Transient receptor potential vanilloid (TRPV) channels are a group of six polymodal cation channels subdivided into two subgroups by their sequence identity and functional properties. TRPV1–TRPV4 comprise the first subgroup of non-selective Ca2+ channels, TRPV5 and TRPV6 constitute the second subgroup of Ca2+ selective channels. TRPV channels are blocked by ruthenium red (RR), a universal pore blocker for a wide array of cation channels. Here we use cryo-electron microscopy to reveal the molecular details of RR block in TRPV2 and TRPV5, members of the two TRPV subfamilies.

Next, we prepared cryo-EM grids of wild-type rat TRPV2 reconstituted into nanodiscs in the presence of 1 mM of the robust TRPV2 activator 2-APB and 1 mM RR. Therefore, we used a high concentration of RR to ensure saturation. This dataset yielded a single stable high-quality state: 2-APB-activated RR-blocked TRPV2 (TRPV22APB+RR) with C4 symmetry at 2.9 Å resolution. The strong extra density at the TRPV22APB+RR SF was clearly visible from early stages of data processing before application of any symmetry and is aligned along the central symmetry axis; the size and shape of this density is consistent with the expected dimensions for RR and density consistent with 2-APB is present at our previously proposed 2-APB binding site and not in the vanilloid pocket (Pumroy et al, 2022). The SF of TRPV22APB+RR has adapted to accommodate RR, with tight coordination by the backbone carbonyl of Gly606 along the interior of the SF and the lower gate is closed at Met645. The primary site for RR stabilization in TRPV22APB+RR is the carbonyl of Gly606, which at distances of 3.0–3.2 Å can form hydrogen bonds with ammonia groups coordinated to the central and bottom ruthenium atoms. Additionally, density for the top ruthenium atom was more poorly resolved than the lower two ruthenium atoms, indicating that the top ruthenium group is not tightly coordinated. The only significant conformational difference between TRPV22APB+RR and TRPV22APB_AC is at the pore, where a downward rotation (9°) and shift (1.1 Å) of the pore helix to accommodate RR leads to subtle shifts in S5 and S6 which constrict the lower gate at Met645. The rest of the channel maintained the previously observed activated conformation, where the C-terminus is in a helical conformation rather than the loop conformation seen in the inactivated state (Pumroy et al, 2022). Our TRPV22APB+RR structure revealed that binding of RR to the 2-ABP-activated TRPV2 stabilized the channel in an intermediate conformation, preventing ion flow through the occluded SF and closing the lower gate at Met645, but at the same time inhibiting the transition to the inactivated state. This TRPV2 locked in an activated conformation allowed us to resolve clear density for 2-APB in our previously proposed 2-APB binding site, but not in the vanilloid pocket, a recently suggested alternate 2-APB site in mouse TRPV2.

>MTSASSPPAFRLETSDGDEEGNAEVNKGKQEPPPMESPFQREDRNSSPQIKVNLNFIKRPPKNTSAPSQQEPDRFDRDRLFSVVSRGVPEELTGLLEYLRWNSKYLTDSAYTEGSTGKTCLMKAVLNLQDGVNACIMPLLQIDKDSGNPKLLVNAQCTDEFYQGHSALHIAIEKRSLQCVKLLVENGADVHLRACGRFFQKHQGTCFYFGELPLSLAACTKQWDVVTYLLENPHQPASLEATDSLGNTVLHALVMIADNSPENSALVIHMYDGLLQMGARLCPTVQLEEISNHQGLTPLKLAAKEGKIEIFRHILQREFSGPYQPLSRKFTEWCYGPVRVSLYDLSSVDSWEKNSVLEIIAFHCKSPNRHRMVVLEPLNKLLQEKWDRLVSRFFFNFACYLVYMFIFTVVAYHQPSLDQPAIPSSKATFGESMLLLGHILILLGGIYLLLGQLWYFWRRRLFIWISFMDSYFEILFLLQALLTVLSQVLRFMETEWYLPLLVLSLVLGWLNLLYYTRGFQHTGIYSVMIQKVILRDLLRFLLVYLVFLFGFAVALVSLSREARSPKAPEDNNSTVTEQPTVGQEEEPAPYRSILDASLELFKFTIGMGELAFQEQLRFRGVVLLLLLAYVLLTYVLLLNMLIALMSETVNHVADNSWSIWKLQKAISVLEMENGYWWCRRKKHREGRLLKVGTRGDGTPDERWCFRVEEVNWAAWEKTLPTLSEDPSGPGITGNKKNPTSKPGKNSASEEDHLPLQVLQSP[4x]>[2x]AASSLDELVALCKRRGFIFQSSEIYGGLQGVYDYGPLGVELKNNLKQAWWRRNVYERDDMEGLDASVLTHRLVLHYSGHEATFADPMVDNRITKKRYRLDHLLKEQPEEVLKRLYRAMEVEEENLHALVQAMMQAPERAGGAMTAAGVLDPASGEPGDWT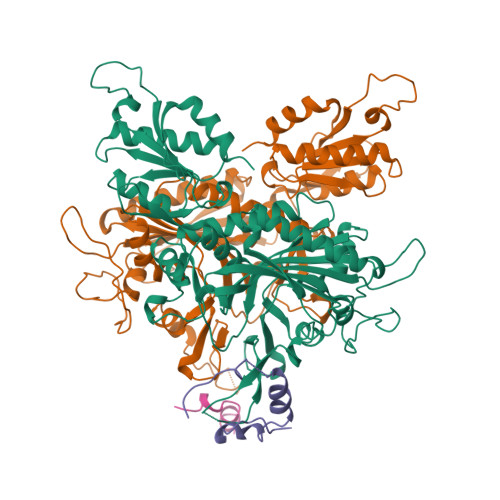PPRYFNMMFQDLRGPRGGRGLLAYLRPETAQGIFVNFKNVLDATSRKLGFGIAQIGKAFRNEITPRNFIFRVREFEQMEIEYFVRPGEDEYWHRYWVEERLKWWQEMGLSRENLVPYQQPPESSAHYAKATVDILYRFPHGSLELEGIAQRTDFDLGSHTKDQEALGITARVLRNEHSTQRLAYRDPETGKWFVPYVIEPSAGVDRGVLALLAEAFTREELPNGEERIVLKLKPQLAPIKVAVIPLVKNRPEITEYAKRLKARLLALGLGRVLYEDTGNIGKAYRRHDEVGTPFAVTVDYDTIGQSKDGTTRLKDTVTVRDRDTMEQIRLHVDELEGFLRERLRW[4-({4-[(5-cyclopropyl-1H-pyrazol-3-yl)amino]quinazolin-2-yl}amino)phenyl]acetonitrile 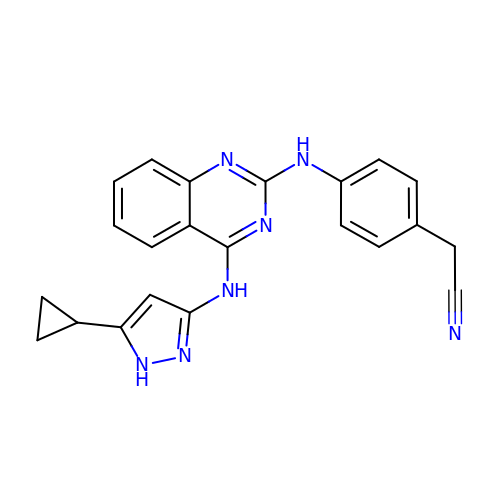| C22 H19 N7 | NVMCVWOODOWOLT-UHFFFAOYSA-N> ANSLVEEFKSGNIERECIEERCSKEEAREVFEDDEKTETFWNVYVDGDQCSSNPCHYRGICKDGIGSYTCTCLSGYEGKNCERVLYKSCRVDNGNCWHFCKHVQNDIQCSCAEGYLLGEDGHSCVAGGNFSCGRNIKTRNKREANLPDF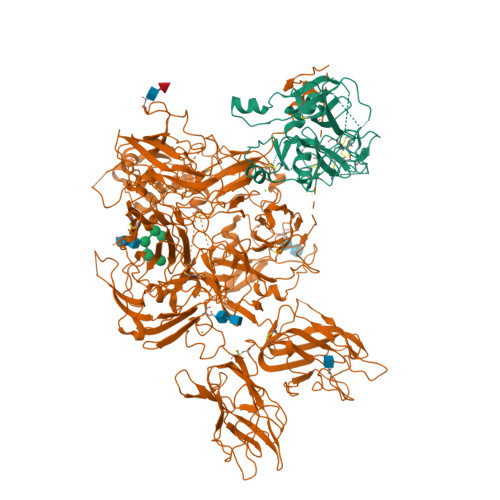VQSQNATLLKKSDNPSPDIRIVNGMDCKLGECPWQAALVDEKEGVFCGGTILSPIYVLTAAHCINETETISVVVGEIDKSRIETGPLLSVDKIYVHKKFVPPQKAYKFDLAAYDYDIAIIQMKTPIQFSENVVPACLPTADFANQVLMKQDFGIVSGFGRIVEKGPKSKTLKVLKVPYVDRHTCMVSSETPITPNMFCAGYDTLPRDACQGDSGGPHTTVYRDTHFITGIVSSGEGCARNGKYGNYTKLSKFIPWIKRIMRQKLPSTESSTGRL;> AQLREYHIAAQLEDWDYNPQPEELSRLSESDLTFKKIVYREYELDFKQEKPRDALSGLLGPTLRGEVGDSLIIYFKNFATQPVSIHPQSAVYNKWSEGSSYSDGTSDVERLDDAVPPGQSFKYVWNITAEIGPKKADPPCLTYAYYSHVNMVRDFNSGLIGALLICKEGSLNANGSQKFFNREYVLMFSVFDESKNWYRKPSLQYTINGFANGTLPDVQACAYDHISWHLIGMSSSPEIFSVHFNGQTLEQNHYKVSTINLVGGASVTADMSVSRTGKWLISSLVAKHLQAGMYGYLNIKDCGNPDTLTRKLSFRELMKIKNWEYFIAAEEITWDYAPEIPSSVDRRYKAQYLDNFSNFIGKKYKKAVFRQYEDGNFTKPTYAIWPKERGILGPVIKAKVRDTVTIVFKNLASRPYSIYVHGVSVSKDAEGAIYPSDPKENITHGKAVEPGQVYTYKWTVLDTDEPTVKDSECITKLYHSAVDMTRDIASGLIGPLLVCKHKALSVKGVQNKADVEQHAVFAVFDENKSWYLEDNIKKYCSNPSAVKKDDPKFYKSNVMYTLNGYASDRTEVLRFHQSEVVQWHLTSVGTVDEIVPVHLSGHTFLSKGKHQDILNLFPMSGESATVTMDNLGTWLLSSWGSCEMSNGMRLRFLDANYDDEDEGNEEEEEDDGDIFADIFIPSEVVKKKEEVPVNFVPDPESDALAKELGLIDDEGNPIIQPRREQTEDDEEQLMKASMLGLRSFKGSVAEEELKHTALALEEDAHASDPRIDSNSARNPDDIAGRYLRTINRGNKRRYYIAAEEVLWDYSPIGKSQVRSRAAKTTFKKAIFRSYLDDTFQTPSTGGEYEKHLGILGPIIRAEVDDVIEIQFKNLASRPYSLHAHGLLYEKSSEGRSYDDKSPELFKKDDAIMPNGTYTYVWQVPPRSGPTDNTEKCKSWAYYSGVNPEKDIHSGLIGPILICQKGMIDKYNRTIDIREFVLFFMVFDEEKSWYFPKSDKSTCEEKLIGVQSLHTFPAINGIPYQLQGLTMYKDENVHWHLLNMGGPKDIHVVNFHGQTFTEEGREDNQLGVLPLLPGTFASIKMKPSKIGTWLLETEVGENQERGMQALFTVIDKDCKLPMGLASGIIQDSQISASGHVGYWEPKLARLNNTGKYNAWSIIKKEHEHPWIQIDLQRQVVITGIQTQGTVQLLQHSYTVEYFVTYSEDGQNWITFKGRHSETQMHFEGNSDGTTVKENHIDPPIIARYIRLHPTKFYNRPTFRIELLGCEVEGCSVPLGMESGAIKNKEITASSYKKTWWSSWEPFLARLNLEGGTNAWQPEVNNKDQWLQIDLQHLTKITSIITQGATSMTTSMYVKTFSIHYTDDNSTWKPYLDVRTSMEKVFTGNINSDGHVKHFFKPPILSRFIRIIPKTWNQYIALRIELFGCEVF>MMSETAPLPSASSALEDKAASAPVV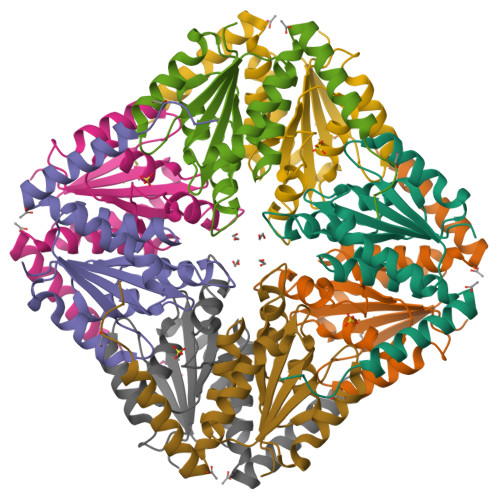GIIMGSQSDWETMRHADALLTELEIPHETLIVVAHRTPDRLADYARTAAERGLNVIIAGAGGAAHLPGMCAAWTRLPVLGVPVESRALKGMDSLLSIVQMPGGVPVGTLAIGASGAKNAALLAASILALFNPALAARLETWRALQTASVPNSPITEDK[2x]>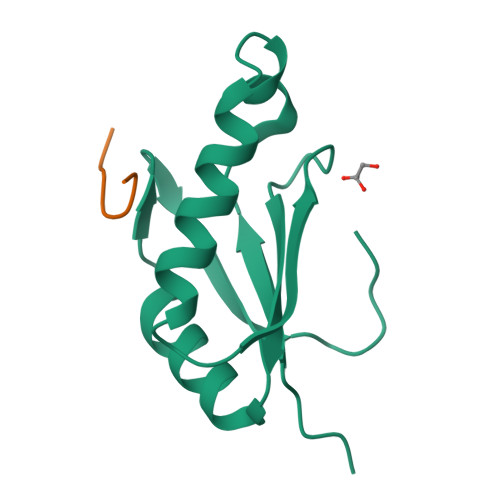 GSMRHERVVIIKNMFHPMDFEDDPLVLNEIREDLRVECSKFGQIRKLLLFDRHPDGVASVSFRDPEEADYCIQTLDGRWFGGRQITAQAWDGTTDY;> NRWDETP> NTYQFRNMIQCTVPSRSWWDFADYGCYCGCGSGTPVDDLDRCCQVHCNCYRQAGEISGCRPKFKTYTYECSGGTLTCKGDNNACAASSCDCDRLAAICFAGAPYNDNNY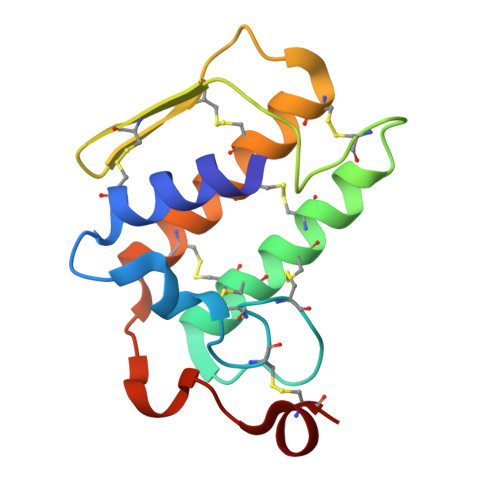NIDLKARCN>[4x]MGSDKIHHHHHHENLYFQGKDYQVAMFGIKSDGVTLNTRSIQRAVDYISEQ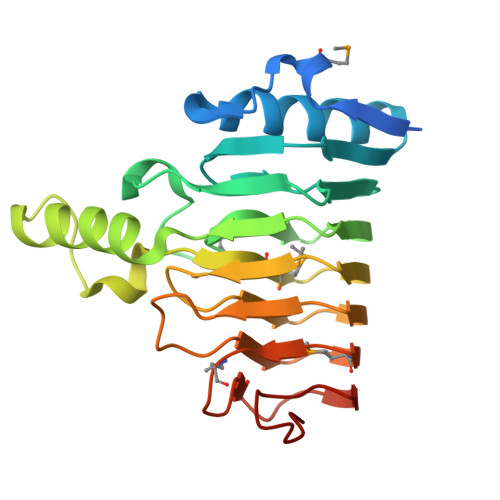GGGRLIFYVGRYLTGSIELKSNVTIRIEEGAVLVAVPSVYDFKGVGGCNAIIYADKQKNIGIGGKGIIDGRSIAVRASVEEQLQKGHIEGNVSDYAPALICMEGCEDVKIEQVTLQDAANVAEIYKDCHNVTVDKVVVNAGASDRKAISISGCDGVKMTDCYFNMAGNPLESAGTSRNLIFTNCITPDGKAVSSDQ> MGHHHHHHSGENLYF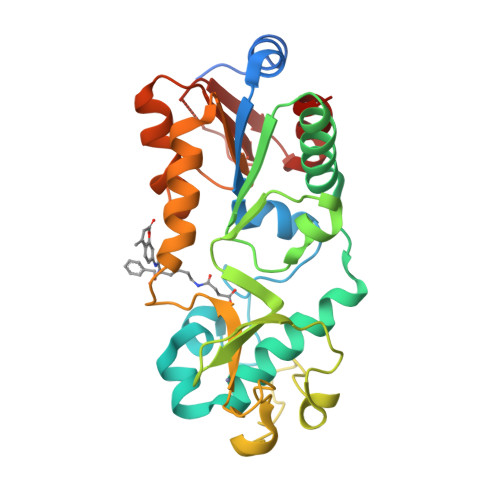QGASARPSSSMADFRKFFAKAKHIVIISGAGVSAESGVPTFRGAGGYWRKWQAQDLATPLAFAHNPSRVWEFYHYRREVMGSKEPNAGHRAIAECETRLGKQGRRVVVITQNIDELHRKAGTKNLLEIHGSLFKTRCTSCGVVAENYKSPICPALSGKGAPEPGTQDASIPVEKLPRCEEAGCGGLLRPHVVWFGENLDPAILEEVDRELAHCDLCLVVGTSSVVYPAAMFAPQVAARGVPVAEFNTETTPATNRFRFHFQGPCGTTLPEALA> EN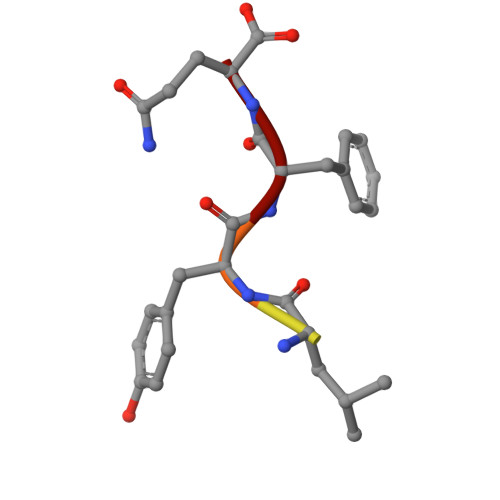LYFQ>[2x]MGHHHHHHHHHHSSGHIEGRHMAAHQLSDFQRNKILRVFNTFYDCNHDGVIEWDDFELAIKKICNLHSWPTDGKKHNEARADLKLIWDGLRKYADENEDEQVTKEEWLKMWAECVKSVEKGE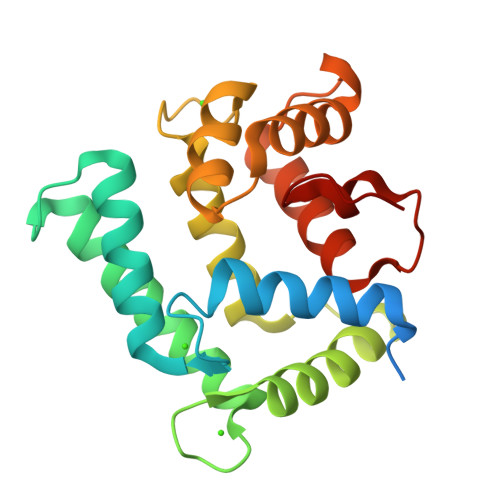SLPEWLTKYMNFMFDVNDTSGDNIIDKHEYSTVYMSYGIPKSDCDAAFDTLSDGGKTMVTREIFARLWTEYFVSNDRGAKGNHLFGTLKL>GMLESTKQFLKKYNINDRVLKLYETAMNDIQNQFKILDDIREFNQLKVLNAFQEERISEAHFTNSSGYGYGDIGRDSLDAVYARVFNTESALVRPHFVNGTHALGAALFGNLRPGNTMLSVCGEPYDTLHDVIGITENSNMGSLKEFGINYKQVDLKEDGKPNLEEIEKVLKEDESITLVHIQRSTGYGWRRALLIEDIKSIVDCVKNIRKDIICFVDNCYGEFMDTKEPTDVGADLIAGSLIKNIGGGIAPTGGYLAGTKDCIEKTSYRLTVPGIGGECGSTFGVVRSMYQGLFLAPHISMEA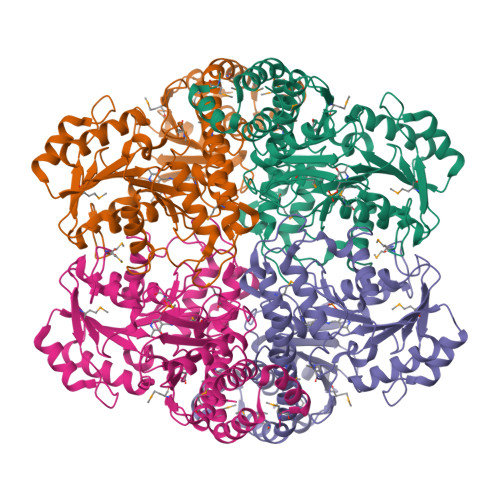LKGAILCSRIMELAGFEVMPKYDEKRSDIIQSIKFNDKDKLIEFCKGIQTGSPIDSFVSCEPWDMPGYTDQVIMAAGAFIQGSSIELSADAPIREPYIAYLQGGLTFDHAKIGILIALSRIVK[4x]~{N}-[4-[4-[(azanylidene-$l^{4}-azanylidene)amino]phenyl]-1,3-thiazol-2-yl]-2-[1,3-dimethyl-2,6-bis(oxidanylidene)purin-7-yl]ethanamide 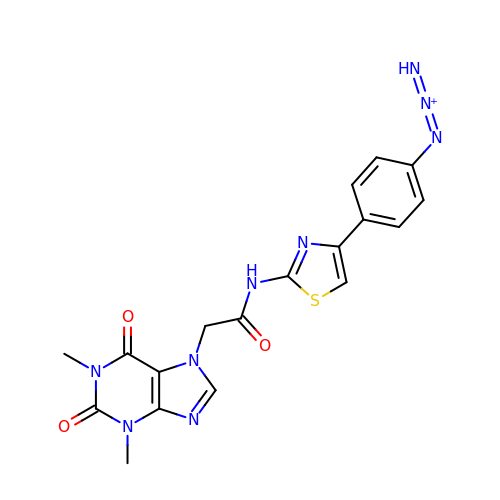| C18 H16 N9 O3 S | BCMLFCZGHWVERY-UHFFFAOYSA-O> EGRMRVLGIETSCDETAVAVLDDGKNVVVNFTVSQIEVHQKFGGVVPEVAARHHLKNLPILLKKAFEKVPPETVDVVAATYGPGLIGALLVGLSAAKGLAISLEKPFVGVNHVEAHVQAVFLANPDLKPPLVVLMVSGGHTQLMKVDEDYSMEVLGETLDDSAGEAFDKVARLLGLGYPGGPVIDRVAKKGDPEKYSFPRPMLDDDSYNFSFAGLKTSVLYFLQREKGYKVEDVAASFQKA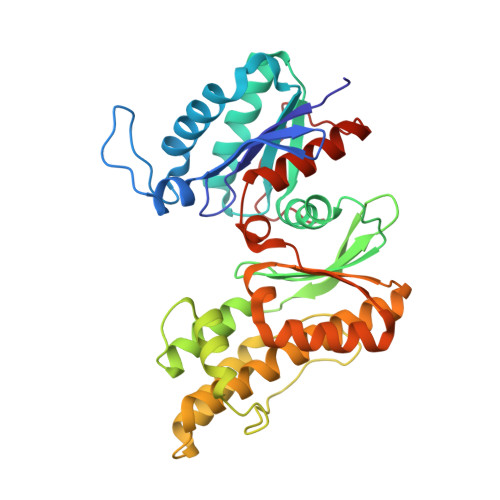VVDILVEKTFRLARNLGIRKIAFVGGVAANSMLREEVRKRAERWNYEVFFPPLELCTDNALMVAKAGYEKAKRGMFSPLSLNADPNLNV>[3x]GSHMGNRRTVTLRRQPVGGLGLSIKGGSEHNVPVVISKIFEDQAADQTGMLFVGDAVLQVNGIHVENATHEEVVHLLRNAGDEVTITVEYLREAPGSAYTNFDAERDALNIETAIKTKGVDEVTIVNILTNRSNEQRQDIAFAYQRRTKKELASALKSALSGHLETVILGLLKTPAQYDASELKASMKGLGTDEDSLIEIICSRTNQELQEINRVYKEMYKTDLEKDIISDTSGDFRKLMVALAKGRRA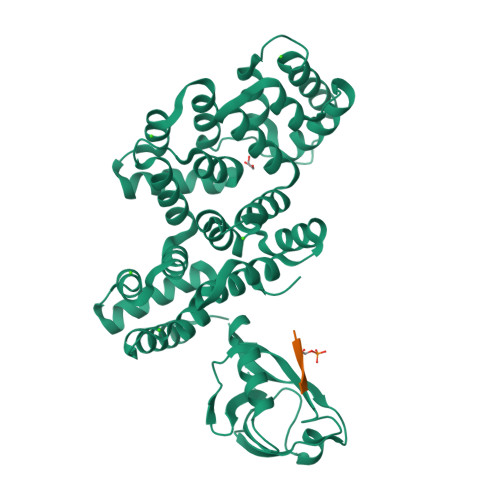EDGSVIDYELIDQDARDLYDAGVKRKGTDVPKWISIMTERSVPHLQKVFDRYKSYSPYDMLESIRKEVKGDLENAFLNLVQCIQNKPLYFADRLYDSMKGKGTRDKVLIRIMVSRSEVDMLKIRSEFKRKYGKSLYYYIQQDTKGDYQKALLYLCGGDD;>RRVRKLPSTTL[3x]>SNAIRPTIGQQMETGDQRFGDLVFRQLAPNVWQHTSYLDMPGFGAVASNGLIVRDGGRVLVVDTAWTDDQTAQILNWIKQEINLPVALAVVTHAHQDKMGGMDALHAAGIATYANALSNQLAPQEGMVAAQHSLTFAANGWVEPATAPNFGPLKVFYPGPGHTSDNITVGIDGTDIA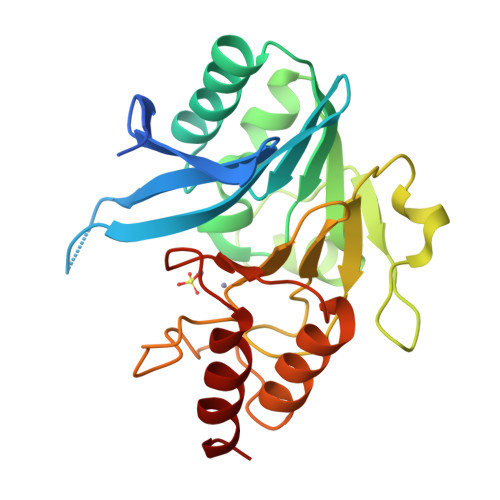FGGCLIKDSKAKSLGNLGDADTEHYAASVRAFGAAFPKASMIVMSHSAPDSRAAITHTARMADKLR[2x]>[4x]MRGSHHHHHHGSMTRSALVTGITGQDGAYLAKLLLEKGYRVHGLVARRSSDTRWRLRELGIEGDIQYEDGDMADACSVQRAVIKAQPQEVYNLAAQSFVGASWNQPVTTGVVDGLGVTHLLEAIRQFSP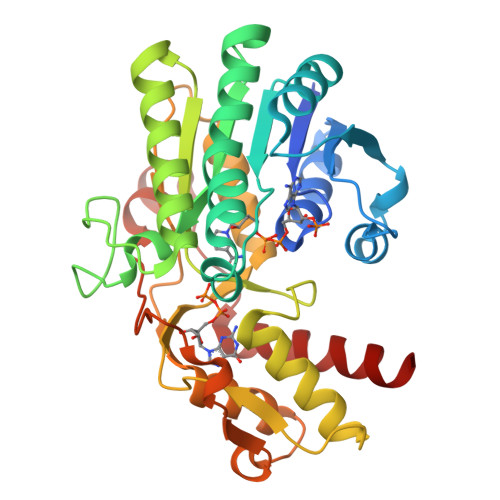ETRFYQASTSEMFGLIQAERQDENTPFYPRSPYGVAKLYGHWITVNYRESFGLHASSGILFNHESPLRGIEFVTRKVTDAVARIKLGKQQELRLGNVDAKRDWGFAGDYVEAMWLMLQQDKADDYVVATGVTTTVRDMCQIAFEHVGLDYRDFLKIDPAFFRPAEVDVLLGNPAKAQRVLGWKPRTSLDELIRMMVEADLRRVSRE>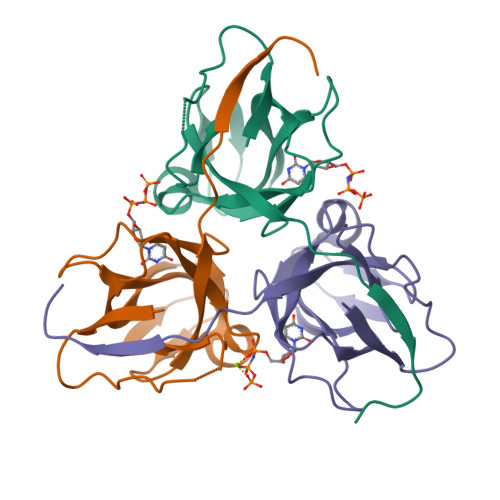[6x]MQIKIKYLDETQTRINKMEQGDWIDLRAAEDVAIKKDEFKLVPLGVAMELPEGYEAHVVPRSSTYKNFGVIQTNSMGVIDESYKGDNDFWFFPAYALRDTKIKKGDRICQFRIMKKMPAVDLIEVDRLGNGDRGGHGSTGTK> ATVQSPDGNIKIIISDEQSTPSYSISFKNKTVINNSALGFEFKQHAPFSNSFKITKVQQQSTNTQWQQPWGERQTVVDQHNEVTVTFAKPQPQGGTYSVRFKAFDSGVGFRYEVPKQAGLNNIEITKELTEFAVNNSHTATAWWIPARGWNKYEYVYNTTPLNDAALVHTPFTFKNQDGVHISIHEAALVDYAAMVLNQRRPGVFQADLTPWSSGVAVKKQGAFNTPWRTIQIGEKAVDLVNSDIILNLNEPNKLGDVSWVKPGKYIGIWWGMHINTHTWGSGDKHGATTKNTKYYMDFAAKYGFDGVLVEGWNTGWDGDWFFNGDVFSFTQPYDDFDIAALTKYSKQTGVQLIGHHETSGNVSNYRKQMADAFALYEKSNVSQVKTGYVADGGNIKRIDKNGIARHEWHDGQFMVNEYLHNVKLAAKHKISINTHEPIKDTGLRRTYPNWITREGARGQEFNAWGTPPNPPEHISMLAFTRMLAGPMDFTPGIFDLSFNGLGANTNRPQTTLAKQLALYVVLYSPIQMAADLPKNYLAK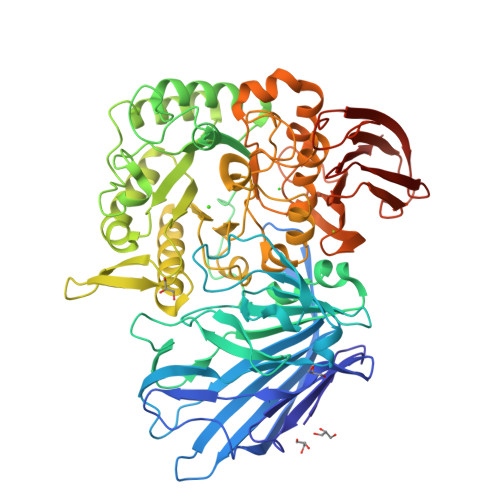PDAFQFIQDVPTDWQQSIALDGAVGDFIVFARKERKRDKYTGNDWYLGAVTDEQARTIEISLDFLDNGKQFEAHIYKDGKNAEWKNNPYDLTIEKRLVTASDKLTLKLATSGGTAIRFKALLEHHHHHH> FQQLSARLQEAIGRLRGRGRITEEDLKATLREIRR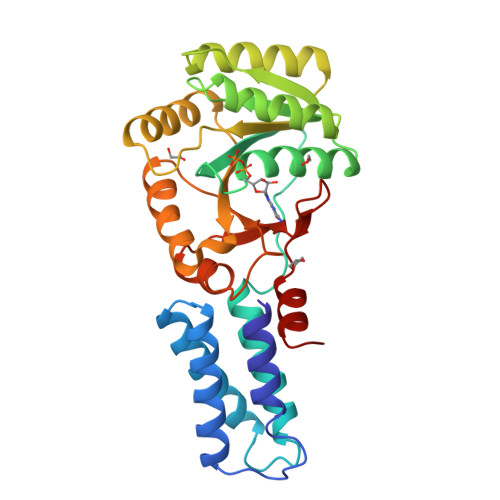ALMDADVNLEVTRDFVERVREEALGKQVLESLTPAEVILATVYEALKEALGGEARLPVLKDRNLWFLVGLQGSGKTTTAAKLALYYKGKGRRPLLVAADTQRPAAREQLRLLGEKVGVPVLEVMDGESPESIRRRVEEKARLEARDLILVDTAGRLQIDEPLMGELARLKEVLGPDEVLLVLDAMTGQEALSVARAFDEKVGVTGLVLTKLDGDARGGAALSARHVTGKPIYFAGVSEKPEGLEPFYPERLAGRILGM> GNLSD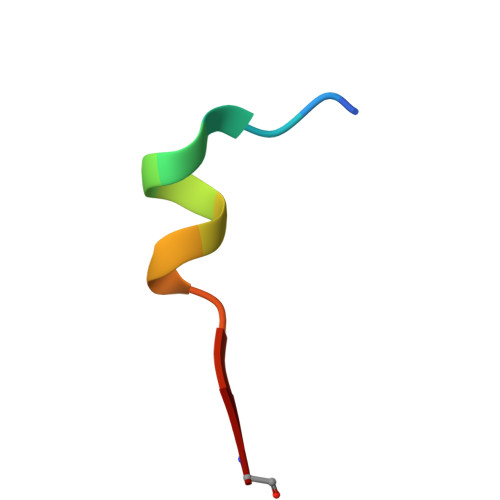DELEGVAGG1-(2,2'-bithiophen-5-yl)methanamine 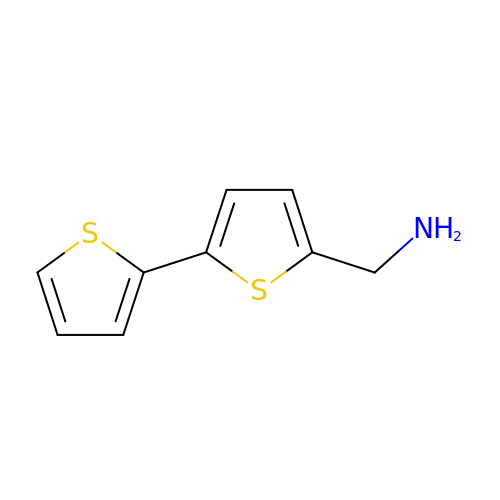| C9 H9 N S2 | FHYTVXBZSXZMGD-UHFFFAOYSA-N> QYSSNTQQGRTSIVHLFEWRWVDIALECERYLAPKGFGGVQVSPPNENVAIHNPFRPWWERYQPVSYKLCTRSGNEDEFRNMVTRCNNVGVRIYVDAVINHMCGNAVSAGTSSTCGSYFNPGSRDFPAVPYSGWDFNDGKCKTGSGDIENYNDATQVRDCRLSGLLDLALGKDYVRSKIAEYMNHLIDIGVAGFRI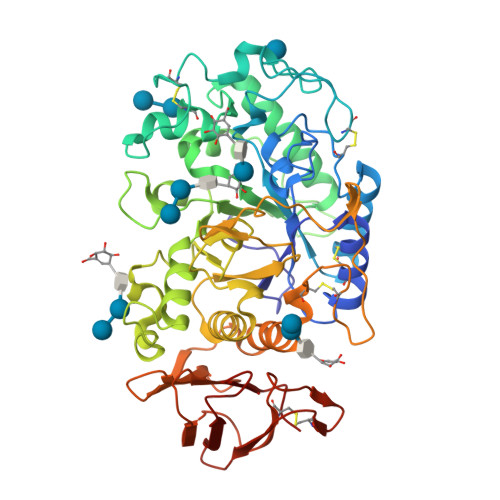DASKHMWPGDIKAILDKLHNLNSNWFPEGSKPFIYQEVIDLGGEPIKSSDYFGNGRVTEFKYGAKLGTVIRKWNGEKMSYLKNWGEGWGFMPSDRALVFVDNHDNQRGHSILTFWDARLYKMAVGFMLAHPYGFTRVMSSYRWPRYFENGKDVNDWVGPPNDNGVTKEVTINPDTTCGNDWVCEHRWRQIRNMVNFRNVVDGQPFTNWYDNGSNQVAFGRGNRGFIVFNNDDWTFSLTLQTGLPAGTYCDVISGDKINGNCTGIKIYVSDDGKAHFSISNSAEDPFIAIHAESKL> NNKTLAAMKNFAEQYAKRTDTYFCSDLSVTAVVIEGLARHKEELGSPLCPCRHYEDKEAEVKNTFWNCPCVPMRERKECHCMLFLTPDNDFAGD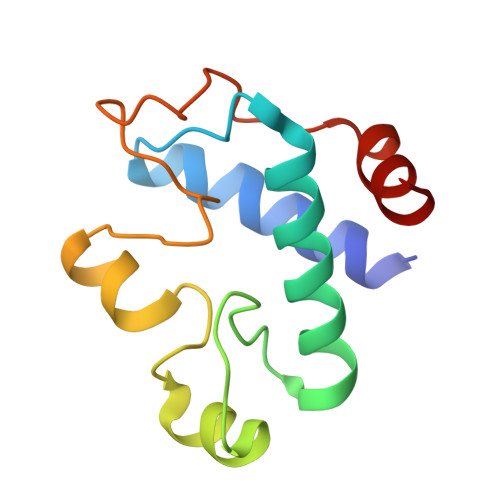AQDIPMETLEEVKAS> GSMSEDIRRGPGRPPKKRVVPNFERKGILEKPVRPQSRLEFSYDNPLIFKNLFIYFKNLKSKNILVRCTPTEITFFSRDQSQASFVIATIDGKNVNHYYASDVFWLGINRELVEKMFNSIDRSFLKITIVHRYDKPETLFFIFTDFDIDKECTYQITVSEPELDMDLIEMEKSISEERLKNYPLRWEFTSKQLKKTFSDLSNYTELVTIEKLGGDTPLHLYFQKFNSISYHEMYKSSNKINLTSTIPKSQVFQINVKIAHIKSLASAMVTDKIRILCEENGNLIFQSEMDALMLNTITLNNTI

AsfvPCNA is a hypothetic sliding clamp family protein; it is coded by the E301R gene that is highly conserved in ASFV strains. The crystal structures were determined at atomic resolution and confirmed that AsfvPCNA can assemble into a homotrimeric ring-shaped structure. Different from homologous protein structures, AsfvPCNA has a very unique amino acid sequence and conformation at the IDCL, J-loop, and P-loop regions, which are involved in partner recognition by PCNAs. Although the detailed molecular basis remains to be investigated, AsfvPCNA has a high dsDNA-binding affinity and can enhance the catalytic activity of the AsfvLIG protein, which plays critical roles in both DNA replication and DNA repair pathways of ASFV.

Using the purified AsfvPCNA protein, we performed extensive crystallization trials and solved the structures in two different forms, Form I and Form II. Form I structure was refined at higher resolution (2.2 Å); therefore, it was used for detailed structural analysis. Form I crystal belongs to P63 space group, per asymmetric unit contains one AsfvPCNA molecule. Out of the total 301 residues of AsfvPCNA, residues 4–15 at the N-terminus and residues 298–301 at the very C-terminus are disordered. The remaining residues form 8 α-helices and 18 β-strands, assembled into two domains, Domain I and Domain II. Domain I (residues 1–155) is composed of α1–3 and β1–9, and Domain II (residues 181–301) consisted of α6–8 and β10–18. Although the side chains of some AsfvPCNA IDCL residues are flexible, the main chains of the IDCL linker are well ordered in Form I structure, supported by the clear 2Fo−Fc electron density maps. In addition to the loop structures at its two ends, AsfvPCNA IDCL also contains two short α-helices, α4 and α5, which are formed by residues 164–171 and 174–177, respectively. Via symmetric operation, Form I AsfvPCNA structure can also form homotrimer. Although it is ordered in the 7DRH structure, the four residues (298NNTI301) are all disordered in the Form I and Form II AsfvPCNA structures, suggesting that AsfvPCNA C-tail is very flexible and can undergo large conformational changes in solution.1-(morpholin-4-yl)-2-[4-(2-{[5-(pyridin-3-yl)-1,3-thiazol-2-yl]amino}pyridin-4-yl)piperazin-1-yl]ethanone 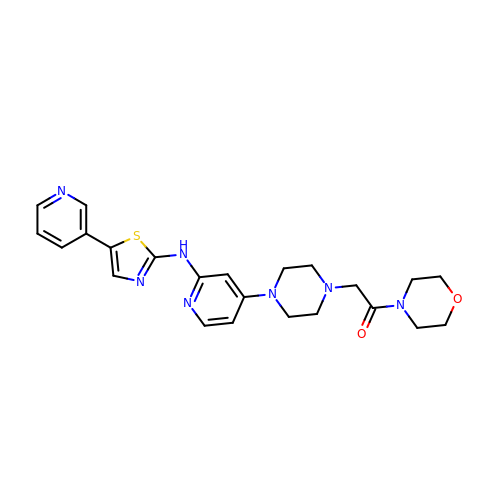| C23 H27 N7 O2 S | QCBHCZCWZWNPGE-UHFFFAOYSA-N> MEKVFYVTTPIYYVNAEPHLGHAYTTVVADFLARWHRLDGYRTFFLTGTDEHGETVYRAAQAAGEDPKAFVDRVSGRFKRAWDLLGIAYDDFIRTTEERHKKVVQLVLKKVYEAGDIYYGEYEGLYCVSCERFYTEKELVEGLCPIHGRPVERRKEGNYFFRMEKYRPWLQEYIQENPDLIRPEGYRNEVLAMLAEPIGDLSISRPKSRVPWGIPLPWDENHVTYVWFDALLNYVSALDYPEGEAYRTFWPHAWHLIGKDILKPHAVFWPTMLKAAGIPMYRHLNVGGFLLGPDGRKMSKTLGNVVDPFALLEKYGRDALRYYLLREIPYGQDTPVSEEALRTRYEADLADDLGNLVQRTRAMLFRFAEGRIPEPVAGEELAEGTGLAGRLRPLVRELKFHVALEEAMAYVKALNRYINEKKPWELF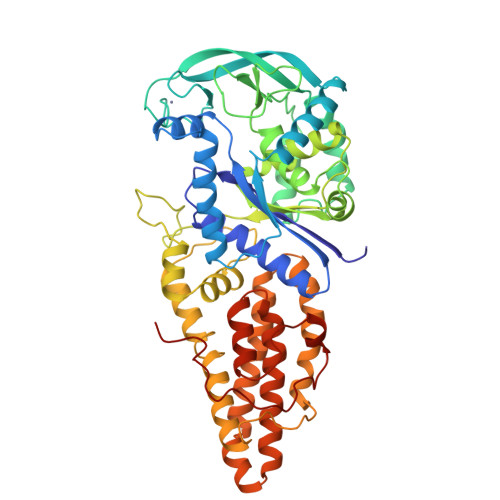KKEPEEARAVLYRVVEGLRIASILLTPAMPDKMAELRRALGLKEEVRLEEAERWGLAEPRPIPEEAPVLFPKK> MQFFK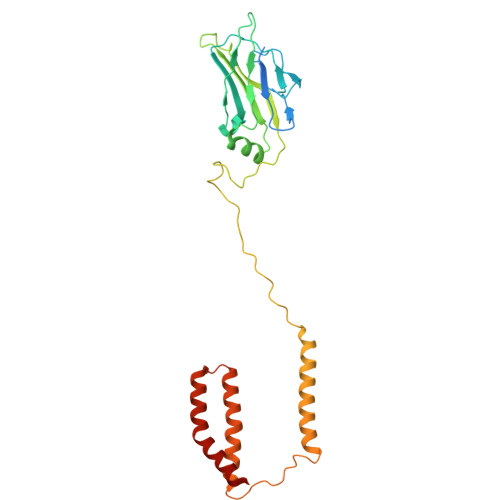TLAALVSCISFVLAYVAQDVHVSFPSTAGKSRVMIGKVEPRIGIDETVPTTITVEDPNEVIQVNFAIESTNKPFQNTLLIGLPNKNLEMAFEPEIKDNGKLSMYKYRIDLAKLDAALLQEASRSPEPIKATLILASSTAKPKENLFREILQLNLNFDVDHSDSSLVDKFGIKPEIHHIFHAEPKRVAKPIAVIFVLIIFITILSLIVTWLNSCAAAFNNIPTGVTAVYFLGFIATIVGFEVIFARYYLGTSIFETLFSSLYLGAPGLLTSTKFLRSFGTI>MKKQFATMLAATAVLGVTTAFAANPFSDVTPDSWAYQAVSQLAQAGIVNGYPDGTFKGQNNITRYEMAQMVAKAMANQDRANAEQQAMINRLADEFSNELNNLGVRVSRLEDRVGNVKVTGDARIRYQGSEDKGVYKANSKSLTDGRARVQFNANVNDKTQAVVRVKGNYEFGDSTKGSQATIDRAYVDHKFGSNVSAKAGRFQQTIGGGLMYDDTFDGAQLNVGNDKVQVQGAYGYMIDGAADGNSKSDNPSVSYVGLKGKVGKESSVGGFYSRLSSGNLNHNGVTVNSDKQDVYGFNADFRKNKLWAGGEWLKASNVDNSQAWTAGLGYGNYDIAKKGTWDVKGQYFNQKANAPIVSSTWDQAYDLTNTSNGYKGYMASVDYAVQ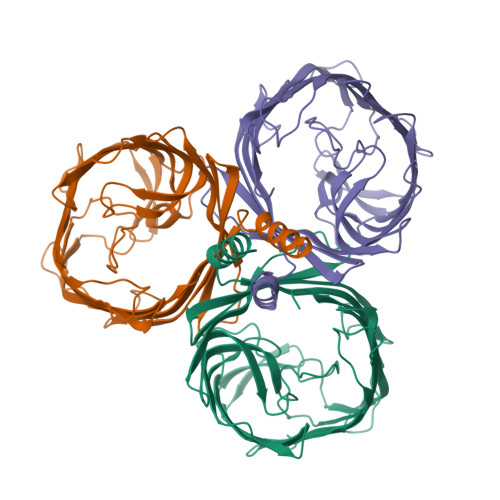DNVGLSAGYGFNSKDQSGNDLSDFYRAELNYKFGGHHHHHH[3x]>[2x]MSLENIMTLPKIKHVRAWFIGGATAEKGAGGGDYHDQGGNHWIDDHIATPMSKYRDYEQSRQSFGINVLGTLIVEVEAENRQTGFAVSTAGEMGCFIVEKHLNRFIEGKCVSDIKLIHDQMLGATMYYSGSGGLVMNTISCVDLALWDLFGKVVGLPVYKLLGGAVRDEIQFYATGARPDLAKEMGFIGGKMPTHWGPHDGDAGIRKDAAMVADMREKCGPDFWLMLDCW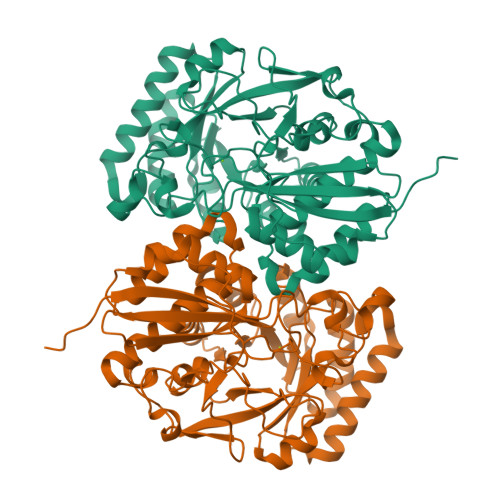MSQDVNYATKLAHACAPFNLKWIEECLPPQQYEGYRELKRNAPAGMMVTSGEHHGTLQSFRTLAETGIDIMQPDVGWCGGLTTLVEIAALAKSRGQLVVPHGSSVYSHHAVITFTNTPFSEFLMTSPDCSTLRPQFDPILLDEPVPVNGRIHKSVLDKPGFGVELNRDCHLKRPYSHEGHHHHHH>RDLYYNDDYVSFLVNTVWKITKPVHIVDYGCGYGYLGLVLMPLLPEGSKYTGIDSGETLLAEARELFRLLPYDSEFLEGDATEIELNDKYDIAICHAFLLHMTTPETMLQKMIHSVKKGGKIICFEPHWISNMASY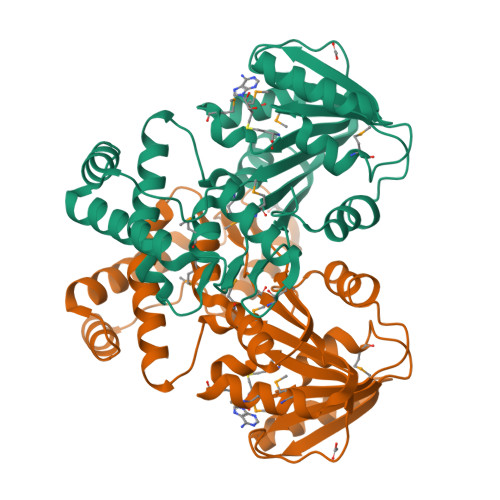LLDGEKQSEFIQLGVLQKLFESDTQRNGKDGNIGMKIPIYLSELGVKNIECRVSDKVNFLDSNMHHNDKNDLYQSLKEEGIAGDPGDKQQFVERLIARGLTYDNALAQYEAELRFFKALHLHSSLVYAPNMKITFGEIECLEHHHHHH[2x]>GSTGGVQTVTLIPGDGIGPEISAAVMKIFDAAKAPIQWEERNVTAIQGPGGKWMIPSEAKESMDKNKMGLKGPLKTPIAAGHPSMNLLLRKTFDLYANVRPCVSIEGYKTPYTDVNIVTIRENTEGEYSGIEHVIVDGVVQSIKLITEGASKRIAEFAFEYARNNHRSNVTAVHKANIMRMSDGLFLQKCREVAESCKDIKFNEMYLDTVCLNMVQDPSQFDVLVMPNLYGDILSDLCAGLIGGLGVTPSGNIGANGVAIFESVHGTAPDIAGKDMANPTALLLSAVMMLRHMGLFDHAARIEAACFATIKDGKSLTKDLGGNAKCSDFTEEICRRVKDLD[4x];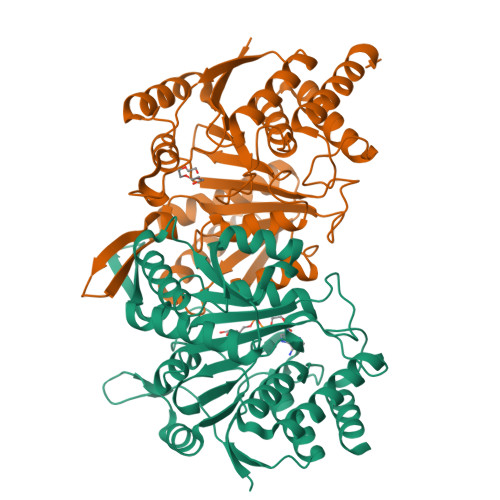>[4x]ASRSQAEDVRVEGSFPVTMLPGDGVGPELMHAVKEVFKAAAVPVEFQEHHLSEVQNMASEEKLEQVLSSMKENKVAIIGKIHTPMEYKGELASYDMRLRRKLDLFANVVHVKSLPGYMTRHNNLDLVIIREQTEGEYSSLEHESARGVIECLKIVTRAKSQRIAKFAFDYATKKGRGKVTAVHKANIMKLGDGLFLQCCEEVAELYPKIKFETMIIDNCCMQLVQNPYQFDVLVMPNLYGNIIDNLAAGLVGGAGVVPGESYSAEYAVFETGARHPFAQAVGRNIANPTAMLLSASNMLRHLNLEYHSSMIADAVKKVIKVGKVRTSDMGGYATCHDFTEEICRRVKDLDENLYFQ>[10x]GSHMGGIEVLDVKTGDDSITQIEAFLNPRMGVNDETNTWYGFSEQVTVATARETDRPPKEQMPYYSCARIPLPLLNEDMTCNTLLMWEAVSVKTEVIGSNTLMNVHDYMTRTDNGVGHPVVGSTYHMFAVGGEPLDLQGIQQSHLVQYPEGLIVPKSVTDVTAKIQCLDPSAKAKLDKDGKYPIETWSPDPSRNENTRYFGNYYGGLTTPPVLTFTNTVTTILL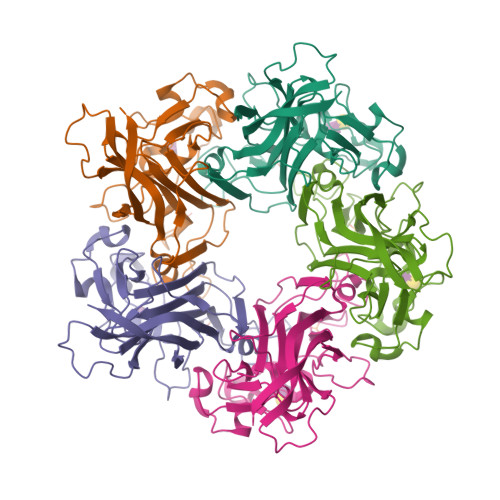DENGVGPLCKGDGLFLSCCDVMGWFTAGSGTHQRFRGLPRYFNVQLRKRAVRN> EPASTLEGPSRPVTVPLREDRGHAVDLPDTDPRVQRRVTGWAPEQIAVALSAAPTSAWVSWITGDFQMGGAVKPLDPGTVGSVVRYGLAADSLVREATGDALVYSQLYPFEGLQNYTSGIIHHVRLQGLEPGTKYYYQCGDPSIPGAMSAVHAFRTMPAVGPRSYPGRIAVVGDLGLTYNTTSTVEHMASNQPDLVLLLGDVSYANLYLTNGTGTDCYSCSFAKSTPIHETYQPRWDYWGRYMEPVTSSTPMMVVEGNHEIEQQIGNKTFAAYSARFAFPSMESESFSPFYYSFDAGGIHFIMLAAYADYSKSGEQYRWLEKDLAKVDRSVTPWLVAGWHAPWYSTYKAHYREAECMRVAMEELLYSYGLDIVFTGHVHAYERSNRVFNYTLDPCGAVHISVGDGGNREKMATTHADDPGRCPEPMSTPDAFMGGFCAF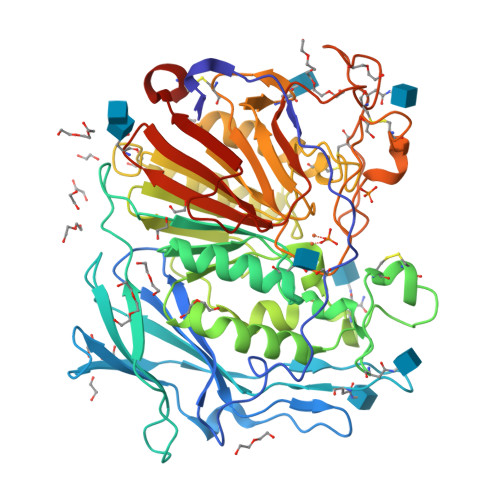NFTSGPAAGSFCWDRQPDYSAYRESSFGHGILEVKNETHALWKWHRNQDLYQGAVGDEIYIVREPERCLLKHHHHHH> APQECSDIAFLIDGSGSIIPHDFRRMKEFVSTVMEQLKKSKTLFSLMQYSEEFRIHFTFKEFQNNPNPRSLVKPITQLLGRTHTATGIRKVVRELFNITNGARKNAFKILVVITDGEKFGDPLGYEDVIPEADREGVIRYVIGVGDAFRSEKSRQE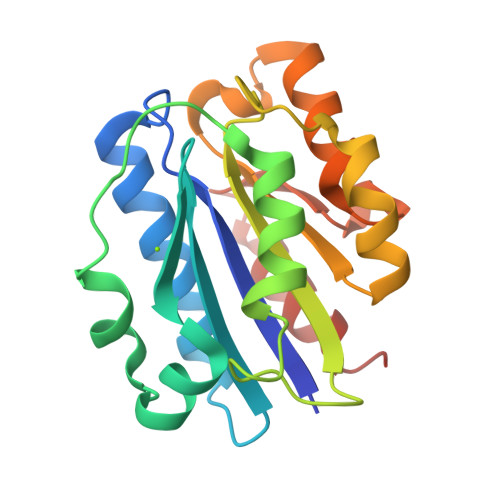LNTIASKPPRDHVFQVNNFEALKTIQNQLRECIFAI>[2x]MRSRRVDVMDVMNRLILAMDLMNRDDALRVTGEVREYIDTVKIGYPLVLSEGMDIIAEFRKRFGCRIIADFKVADIPETNEKICRATFKAGADAIIVHGFPGADS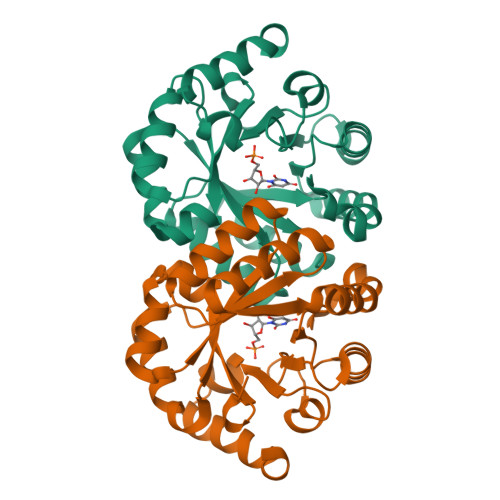VRACLNVAEEMGREVFLLTEMSHPGAEMFIQGAADEIARMGVDLGVKNYVGPSTAPERLSRLREIIGQDSFLISPGVGAQGGDPGETLRFADAIIVGRSIFLADNPAAAAAGIIESIKDLLNP>[32x]MSIVTKSIVNADAEARYLSPGELDRIKAFVTGGAARLRIAETLTGSRETIVKQAGDRLFQKRPDIVSPGGNAYGEEMTATCLRDMDYYLRLVTYGVVSGDVTPIEEIGLVGVREMYRSLGTPIEAVAQSVREMKEVASGLMSSDDAAEASAYFDFVIGKMS;>MQDAITAVINSADVQGKYLDGAAMDKLKSYFASGELRVRAASVISANAATIVKEAVAKSLLYSDVTRPGGNMYTTRRYAACIRDLDYYLRYATYAMLAGDASILDERVLNGLKETYNSLGVPISSTVQAIQAIKEVTASLVGADAGKEMGVYLDYICSGLS[34x];>MSVVSQVILQADDQLRYPTSGELKGIQAFLTTGAQRIRIAETLAENEKKIVDQAQKQLFKKHPEYRAPGGNAYGQRQYNQCLRDYGWYLRLVTYGVLAGNKEPIETTGLIGVKEMYNSLNVPVPGMVDAVTVLKDAALGLLSAEDANETAPYFDYIIQFMS[2x];>[2x]MRDAVTTLIKNYDLTGRYLDRNAMDELKAYFESGSARIAAAAMINANSATIVKRAAAQLFEEIPELIRPSGNAYTTRRFSACLRDMDYYLRYASYALIAADNNVLDERVLQGLRETYNSLGVPIGPTVRGIQIMKEMIEAMAEDSSLNSTDFIASPFDHMTRELSELSV;>MRMFRITACVPSQTRIRTQRELQNTYFTKLVPYDNWFREQQRIMKMGGKIVKVELATGRPGTNAGLA[6x];>[2x]MSVKASGGSSLARPQLYQTVPVSAISQAEQQDRFLEGSELNELTAYFQSGALRLEIAETLTQNADLIVSRAANRIFTGGSPLSYLEKPVERQPALVGASSDSRNGSVTYAESNGSGGLFGGLRSVFSSTGPIPPGFRPINIARYGPSNMQKSLRDMSWFLRYT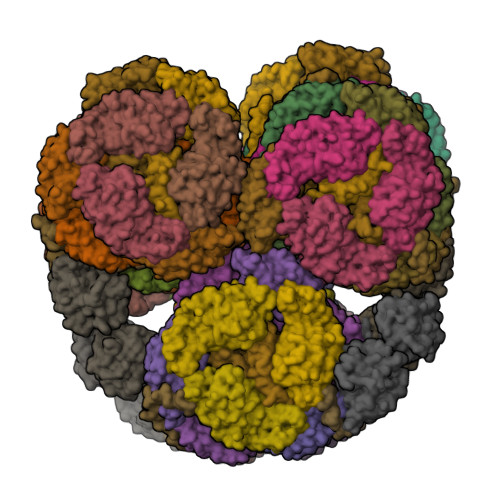TYAIVAGDPNIIVVNTRGLKEVIENACSIDATIVAIQEMRAASADYFRNNAQAKEIVLQYFDILLSEFKAPTPANKVRQGPSNDIQGLELPQSYFNAAAKRQKYAMKPGLSALEKNAVIKAAYRQIFERDITKAYSQSISYLESQVRNGDISMKEFVRRLAKSPLYRKQFFEPFINSRALELAFRHILGRGPSSREEVQKYFSIVSSGGLPALVDALVDSQEYADYFGEETVPYLRGLGVEAQECRNWGMQQDLFSYSAPFRKVPQFITTFAQYDRPLPDQHVYGSGNDPLEIQFGAIFPKETRNPSKRPAPFNKDTKRILIHRGPAVNNQVGNPSAVGEFPGSLGAKVFRLNGGLPGAKVGKNTGTSVKFGESSTQALIRAAYRQVFGRDLYEGQRLSVAEIQLENGDISVREFIKRLAKSELFLKLYWAPHYVCKAIEYMHRRLLGRPTYGRQEMNQYFDIASKQGFYAVVEAMIDSKEYSDAFGEDTVPYERYLTPGGLQMRSARVGSLREDIGQRVDKEVTPRFVELGQVSAIRTEPEIAYRSNQGVTRQRQQTKVFKLVSTYDKVAVKNAIRAAYRQVFERDLEPYIINSEFTALESKLSNNEINVKEFIEGLGTSELYMKEFYAPYPNTKVIEMGTKHFLGRAPLNQKEIQQYNQILASQGLKAFIGAMVNGMEYLQTFGEDTVPYRRFPTLPAANFPNTERLYNKLTKQDKELVVPSFTPVVKVGG;>[2x]MLKKLFGAKKEFYVQLDESQAPAQVEEADVAIVKSEVAPVEKPAPTTSKKTSIKKKSATKAAAPVETPASAPVAPAPKAKVDPSQVAFASGDPIPQNVARRTPGPSLNRFKEMARQVKVKR;>MALPLLNYAPKSQNVRVEGYEIGSEEKPVVFTTENILSSSDMDNLIEAAYRQIFFHAFKWDREKVLESQLRNGQITVRDFVRGLLLSNTFRNSFYEKNSNYRFVEHCVQKILGRDVYSEREKIAWSIVVATKGYQGLIDDLLNSDEYLNNFGYDTVPYQRRRNLPGREAGELPFNIKSPRYDAYHRRQLGFPQIVWQNEVRRFIPQEKKLTAGNPMNFLGMARSINPAANTIPKVSAQNINIEASVPRR[6x];>[4x]MPFTIDSARGIFPNTLAADVVPATIARFSQLNAEDQLALIWFAYLEMGKTLTIAAPGAASMQLAENALKEIQAMGPLQQTQAMCDLANRADTPLCRTYASWSPNIKLGFWYRLGELMEQGFVAPIPAGYQLSANANAVLATIQGLESGQQITVLRNAVVDMGFTAGKDGKRIAEPVVPPQDTASRTKVSIEGVTNATVLNYMDNLNANDFDTLIELFTSDGALQPPFQRPIVGKENVLRFFREECQNLKLIPERGVTEPAEDGFTQIKVTGKVQTPWFGGNVGMNIAWRFLLNPEGKIFFVAIDLLASPKELLNFAR LapG-containing operons also harbor a gene that encodes a conserved c-di-GMP receptor, LapD. LapD is composed of a periplasmic Cache domain, flanked by single-transmembrane helices, followed in the cytoplasm by a juxtamembrane HAMP domain with a signaling (or S) helix that leads into a GGDEF and EAL domain module. However, in LapD, both domains are enzymatically inactive, yet the EAL domain retains its ability to bind c-di-GMP. Through detailed structure-function studies, a mechanism for the regulation of LapG via LapD has emerged: LapD adopts an autoinhibited conformation that is characterized by the GGDEF domain functioning as a lid atop the EAL domain, which occludes the c-di-GMP binding site.

To gain unbiased insight into the structure and regulation of V. cholerae LapD, we determined a crystal structure of its cytoplasmic domains comprising the S helix followed by GGDEF and EAL domains in the absence of c-di-GMP. Crystals diffracted X rays to a maximum resolution of 2.7 Å. The electron density maps resolved the S helix with the final refined model spanning residues 221 to 638 (top). Despite the low sequence identity, the structures of V. cholerae and P. fluorescens LapD superimpose with an overall root mean square deviation (RMSD) of 1.7 Å, indicating structural conservation of their apo states. The major difference pertains to a rigid body rotation of the GGDEF domain of approximately 12° relative to the EAL domain. However, the autoinhibitory S helix-EAL domain interaction responsible for P. fluorescens LapD autoinhibition at low cellular c-di-GMP levels is well preserved in the structure of the V. cholerae ortholog. More specifically, residues F223, A227, and R234 of the S helix (corresponding to F222, A226, and R233 of P. fluorescens LapD) nestle against a partially hydrophobic interface on the EAL domain. As seen with P. fluorescens LapD, this contact places the GGDEF domain atop the putative c-di-GMP binding site on the EAL domain. Based on structural work, we show that the Vibrio cholerae LapD ortholog adopts a similar autoinhibited conformation utilizing the same intramolecular interfaces as determined for the related P. fluorescens LapD, despite low sequence conservation.

>[2x]KAFKAQAKEAQQLRERAYLDPVSHLGNRAYYMSQLSGWLSESGIGGVAILQAEFIKELYEEKGYEAGDGMVRELADRLKNSITIKDISIARISTYEFGIIMPNMDETELKIVAESIITCVDDINPDPTGMAKANLSLGVVSNKRQSSTTTLLSLLDNALAKAKSNPELNYGFISSDTDKIILGKQQWKTLVEEAIHNDWFTFRYQAANSSWGKTFHREVFSAFEKDGVRYTANQFLFALEQLNASHIFDQYVIERVIQQLEKGELTDPLAINIAQGSISQPSFIRWISQTLSKHLSVANLLHFEIPEGCFVNEPHYTALFCNAVRNAGADFGVDNYGRNFQSLDYINEFRPKYVKLDYLFTHHLDDERQKFTLTSISRTAHNLGITTIASRVETQTQLDFLSEHFIEVFQGFIVDKAA> TRDFNGTWEMESNENFEGYMKALDIDFATRKI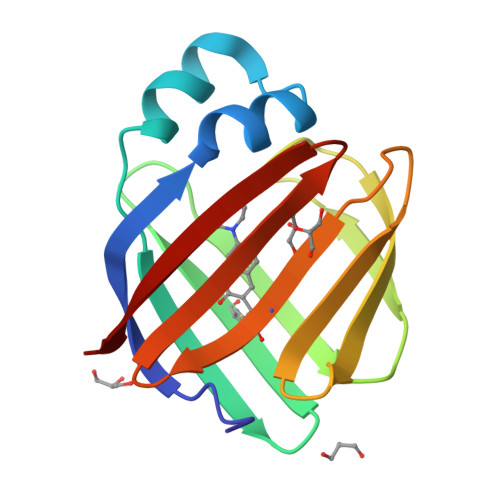AVRLTFTLVIDQDGDNFKCKATSTFLNYDVDFTVGVEFDEYTKSLDNRHVKALVTWEGDVLVCVQKGEKENRGWKKWIEGDKLYLELTCGDQVCRQVFKKK>[6x]MKISDGNWLIQPGLNLIHPLQVFEVEQQDNEMVVYAAPRDVRERTWQLDTPLFTLRFFSPQEGIVGVRIEHFQGALNNGPHYPLNILQDVKVTIENTERYAEFKSGNLSARVSKGEFWSLDFLRNGERITGSQVKNNGYVQDTNNQRNYMFERLDLGVGETVYGLGERFTALVRNGQTVETWNRDGGTSTEQAYKNIPFYMTNRGYGVLVNHPQCVSFEVGSEKVSKVQFSVESEYLEYFVIDGPTPKAVLDRYTRFTGRPALPPAWSFGLWLTTSFTTNYDEATVNSFIDGMAERNLPLHVFHFDCFWMKAFQWCDFEWDPLTFPDPEGMIRRL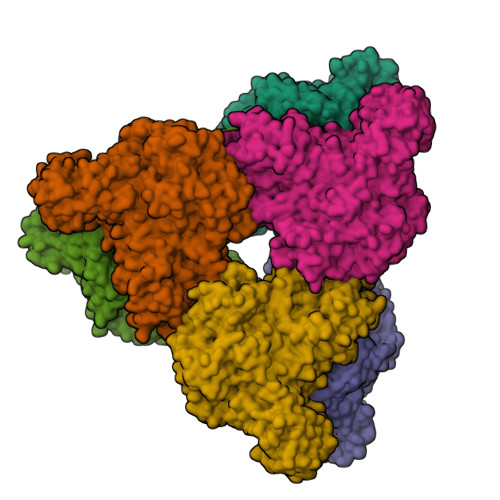KAKGLKICVWINPYIGQKSPVFKELQEKGYLLKRPDGSLWQWDKWQPGLAIYDFTNPDACKWYADKLKGLVAMGVDCFKTDFGERIPTDVQWFDGSDPQKMHNHYAYIYNELVWNVLKDTVGEEEAVLFARSASVGAQKFPVHWGGDCYANYESMAESLRGGLSIGLSGFGFWSHDIGGFENTAPAHVYKRWCAFGLLSSHSRLHGSKSYRVPWAYDDESCDVVRFFTQLKCRMMPYLYREAARANARGTPMMRAMMMEFPDDPACDYLDRQYMLGDNVMVAPVFTEAGDVQFYLPEGRWTHLWHNDELDGSRWHKQQHGFLSLPVYVRDNTLLALGNNDQRPDYVWHEGTAFHLFNLQDGHEAVCEVPAADGSVIFTLKAARTGNTITVTGAGEAKNWTLCLRNVVKVNGLQDGSQAESEQGLVVKPQGNALTITL>MGKVLWDGRAPR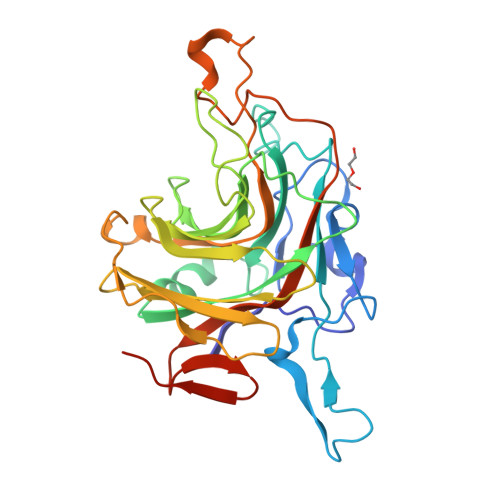NYTSFHLDASVDPYLTVVKGPRAASIYTRLLGREVTPTPLWNDRLFPEVPYPAVSTEQALLVLIGNSSVFTPGSSGRPQTGFRRTELIAQVNGSNIDLIPIIGKGRVAFHFSVLMDEWHKLDMIHEHQLVFVEPSDGSHVFTLQVGSPFTNPTGPLPAPRADWLKILNHNLDVLFETEFTDETWHNFAVIVDWEKRTLQVWYSQNENNLVWVTPVLPNETVKRGTAGRGDFHFGILKLPLVNVADPPEVRDDVVHYGIQPPTTHGIMYSGVFIEDLEDGLSVGNKFIQEVAAALEHHHHHH[2x]(2~{R},3~{R},4~{R},5~{R})-4-[(2~{S},3~{R},4~{S},5~{R},6~{R})-6-(hydroxymethyl)-3,4,5-tris(oxidanyl)oxan-2-yl]oxy-2,3,5,6-tetrakis(oxidanyl)hexanal 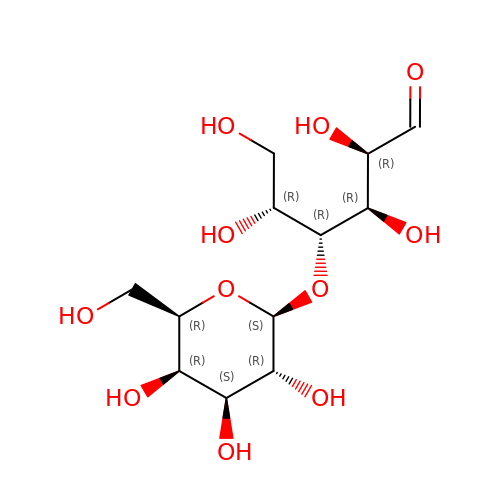| C12 H22 O11 | DKXNBNKWCZZMJT-JVCRWLNRSA-N> ISGGDAIYSSTGRCSLGFNVRSGSTYYFLTAGHCTDGATTWWANSARTTVLGTTSGSSFPNNDYGIVRYTNTTIPKDGTVGGQDITSAANATVGMAVTRRGSTTGTHSGSVTALNATVNYGGGDVVYGMIRTNVCAEPGDSGGPLYSGTRAIGLTSG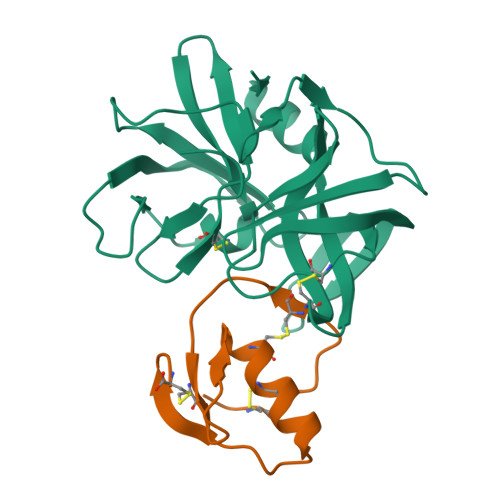GSGNCSSGGTTFFQPVTEALSAYGVSVY;> VDCSEYPKPACTWEYRPLCGSDNKTYGNKCNFCNAVVESNGTLTLSHFGKC STAUROSPORINE | C28 H26 N4 O3 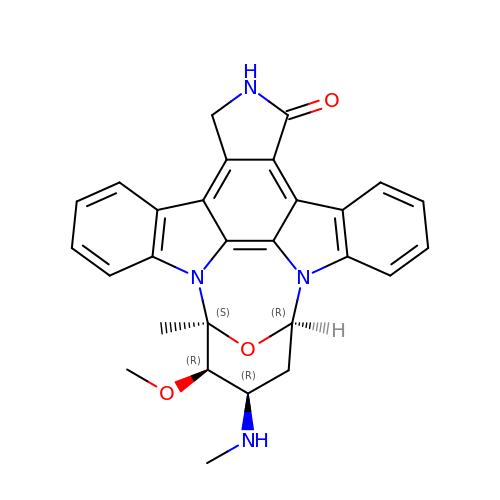| HKSZLNNOFSGOKW-FYTWVXJKSA-N>[7x]MQIQRHSFKWILYGFLCWMTSFVQAQTPTLTNATPAEGFIGEQVCFPVTFVNTGAPGYGPYVRLIVPTGFTFDNASFGGSIQTVQNLGVIVSGAPNNFVIDPIAQSNNNSTTSDTIFAPVGSTVILLEYPVGSMVQGGVSLISEVCMTVDPAATIGVPVDICTQGVYEFGDTPTGDNGPIAGANECEPIIPILFRFDKKVNGSDGVYNEVPGGGASLCHIHQYELNIDIAAAGTLNGPITITDVLPGELAYFGNISLPAGCSAVEPTVGGLGGTLTVTCNGSYPGSTANIDMQVTFDAAVSDTLDETICDDTDINNGATVNVPGNPSQSDTVVTHVEHVLLGHTNNTVSPVTIGQTVLYTIGAEITEYTAGLTAASITFIVPDGMIYNPASLTWAGTPVAAGNVVIVPGPGTGSTVTVDVHTQNGANILPCASPSLQYTADVNQTYANGDPVLSRDRLTHSSTLTYDLVEGATGCTTSAGTPIDVIDIFFQKTVNNSPPTGPGRNGQWWPGDVVQYRLELQIPSLDLDDVVITDFFPLPIHDVASLAATFGTDVRFDPATCWNTAPVTYTRDIPTNSLILDFGDVSDLVTGGCVDIVLLIDIPITTLPFADGLFHSNFMQVNSDNSTADNITNSALTLIQVGAPDLELTKGIVSSDNPNVTISPTVVPPDGNATDVSAGDQLFFDITIENVGGAPGYDVQVRDVAPPELTNCALVAPNPVVDGSNNALAFSGGFVGNTLTIDLVAPNDSIAFATAPNNNDLITVSYVCEAVAGIQAGTRFDNTAEVDWSSTRGGVKFPPVEDDANGRIADPTMNKVVDYIFPNYSNTNTQASIGEVVAYELQLNIPEGNMNNVTLVDQVDEGLAFVAVDSIVICNSSGSTNIITSIGGGFPAVQSGATITNLGANPQQQDRVLTLDFGNLQNLDTDNIEDTIKVYYRTIVINHVTNFDGERVRNRAVLSWDNPNTPGDRSSINDRAPFVTIVEPQLEISKSFTPDEVLPGNNSFVTLTVRNPGTSSAPAFDVSLTDILPTGMTFVSGFSAGGTASITTPPTNGGGTITAHWDTINVGEVYSITFEVQASSSITPCFTLTNCANLVWESIAEADEPNMPTAFSSNLGVQRTGNPGNLGGAANTYTQDSCADLDVVIDNTFDPFITANTPLCEGDRVVLTVQQYQGNVVRYNWTGPGVPAGFNNYELVLDPVTTADTGTYFVYVELDGCITDTSNFFSLQLRPKPVTPNINPGDTTICEGTSIQFSTSTIANDYTWTGPNGFTANSATTPLISPVTLADAGRYTLFTTNAQGCNSDPISSNLTVTPRPAQPSIASNTPICSNENIILTSSTSAITYQWMAPNGQDTITTNNTLTLEPNNPLYTAGNWTLVVFDANGCASQPSTAANVIINGTPIAPMTSNSGPICEGEDVTLMVNTVSSGTYAWYSDANLTNLVASTQNPVISGLLASNSPDTFYVQVSSNGCLSDTGFTVVQVNPNPAAVSPGYTPLCSGDTIFLFANATANIYNWTGPNGFVSNLENPFIANSAALNAGSYTVSITDANGCSNSGIVQVAVDERPVTPTITGNGPVCEGDNIQLNIGSYTGTTVQYTWSTPTGVVTTGVPSLNINNTTVADSGLYSVVVAVDGCTSLADSINIVVRPNPIAPNVPSNFSVCEGDGIALTTTTNANIYNWTGPNGFSSNSPNPTVISPASSANAGTYTLVVQDFNGCTSPAASTVVTVNAAPAQPSMTTNSPICNGADLVMSTSAAGNSYIWRAPNGADTTTASSTLTIVPTSSLYQSGNWTLSVVNAAGCVSPASIASAVEINSIPSTASAGNNGPVCTGTDASLSAGTVSGASYAWYTDAGTSNQFSTLQNPTVNNLTNDSTFYLLVTVNGCPSALDSTTVVVYPLTPSPS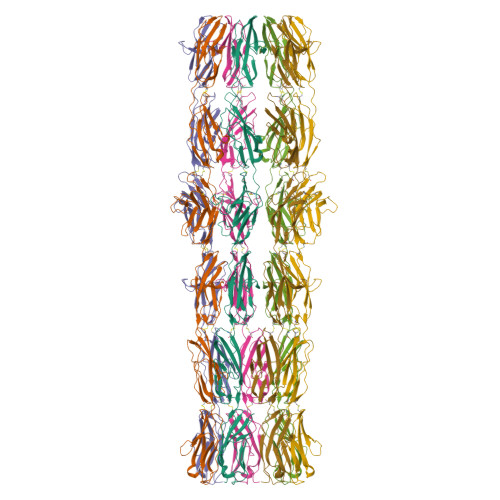LPANFAVCEGDDIALSTSTVASSYDWSGPNGFTSNAQNPVVITNATGSNAGVYTLSIVDGNGCSSADTSVQVTVNAAPTQPSMTTNSPICNGADLVMSTSAVGNSYIWRAPNGADTTTASSTLTIVPTSSLYQSGNWTLSVVNAAGCVSPASIASAVEINSIPSTASAGNNGPVCTGTDASLSAGTVSGASYAWYTDAGTSNQFSTLQNPTVNNLTNDSTFYLLVTVNGCPSALDSTTVVVYPLTPSPSLPADFAVCEGDDIALSTSTVASSYDWSGPNGFTSNAQNPVVITNATGSNAGVYTLSIVDGNGCSSADTSVQVTVNAAPAQPSMTTNSPICNGADLVMSTSATGNSYIWRAPNGADTTTASSTLTIVPTSSLYQSGNWTLSVVNAAGCVSPASIASAVEINSIPSTASAGNNGPVCTGTDASLSAGTVSGASYAWYTDAGTSNQFSTLQNPTVNNLTNDSTFYLLVTVNGCPSALDSTTVVVYPLTPSPSLPADFAVCEGDDIALSTSTVASSYDWSGPNGFTSNAQNPVVITNATGSNAGVYTLSIVDGNGCSSADTSVQVTVNAAPTQPSMTTNSPICNGADLVMSTSAVGNSYIWRAPNGADTTTASSTLTIAPTSSLYQSGNWTLSVVNAAGCVSPASVASMVTINNGTNPTAFNNGPVCRGDAVQLNTTTINNALYEWYSDAALTNLISTQQNPTVANITTDSTFYLVVTVNGCPSSAVATTVTLHPTPATPNIPANFVVCEGETIALSTSTVASSYNWTGPNGFTSNLQNPAVIQPATTADAGSYTLFIVDANGCQSADTSVVVGVNRGPAAPVLTNNSAICDGDTLLLSTTASADTFRWISPNGIDTITTVNSLMIVPTNGTYYQSGDWTLITQVANNCPSEPSAPSSVVINSSTAAPTAFNDGPVCVGGDVTLSTPSAPGAFYQWYTDAALTNLVATTASFTAINITQDSTFYLVVTVNGCTSPAGSTVVNVIGQPSAPNVPADFEVCEGDDIILGTTTIAASYSWTGPNGFTSNLQNPAAITNASLIDSGIYRLVVTYSNGCVSADTTVRVGVNSNPPVPNIVSNGPICFGDTLVLSSSTSCGQSQWIGPNGNSQSTLGTPGGSNVLWTIGSTTSIPMNNANYLPGNWYMICIDTVTGCRSESNTINVIINANPDTPAVFNDGPVCEGGNSNLSTATVSGASYAWYSDSSLTSLVSTAQNPMIVNISTDTTWYLVVTVNGCSSVAGSTTVIVHPTPVTPNVPANFAVCEGDNITLSTSTVASSYNWSGPNGFTSNVQNPVVITNATTSNAGVYTLSIIDGNGCESGDTAVTVTVDSIPATPVLSSNSAICFGDTLELSTTALATSYEWIAPDGSRITTGTNILSISSNNSLYQSGDWMLVTTNASGCTSMPSSVATVVINANPAQPAVFNDGPVCEGGNSNLSTATVSGASYAWYSDSSLTSLVSTAQNPMIVNISTDTTWYLVVTVNGCSSVAGSTTVIVHPTPATPNVPANFAVCEGDNITLSTSTVASSYNWSGPNGFTSNVQNPVVITNATTSNAGVYTLSIVDGNGCESGDTTVTVTVDSIPVTPVLSSNSAICFGDTLELSTTALATSYEWIAPDGSRITTGTNILSISSNNSLYQSGDWMLVTTNASGCTSMPSSVATVVINANPAQPAVFNDGPVCEGGNSNLSTATVSGASYAWYSDSSLTSLVSTAQNPMIVNISTDTTWYLVVTVNGCSSVAGSTTVIVYPTPATPNVPANFAVCEGDNITLSTSTVASGYNWSGPNGFTSNVQNPVVITNATASNAGVYTLSIVDGNGCESGDTTVTVTVNGNPPVATITSNSPICFGDTLTLSSSTNCGQSQWIGPNGNSSGTLGTPGGNNVLWTIGSTTNIPSTDVNYLSGDWYMICIDTITGCRSESNTITIEINPIPVVSAFNNGPICAGEDGELSATFITGASYRWYSDATLTTLISTSRTPIISSMMSSETYYVVATVNGCTSLADSTTIVVNPTPVIPNPTYTPLCQLDTLFLQANAVGPIATYWWTGPNGFTSHLENPVIPNIYPFNAGSYILTVTDSLGCEAVSTVEVTIYPKPQTPTIAHNAPFCEGTNDLTLTTQAYFGTDVRYIWTLPNGNLDTTFVPSLVLPNATVQDTGAYSLVVWIDGCLSLPAEEIIRIYPTPATPNVPADFAVCEGEAIVLTTTTNATSYFWTGPNGFQSNLQSPSVVNATLVDAGSYHLYVTNTWGCQSLDTSVQVTVNANPPIATITSNSPICFGDTLTLSSSTNCGQSQWIGPNGNSTGTLGTPGGNNVLWTIGSTTNIPSTDSNYLSGDWYMICIDTITGCRSESNTITIDINPIPSTPAAFNNGPICIGGTAQLSTTTVSGATYAWYADATLTTLVATNQNPTISNITTDSTFYIVVTVNGCSSLAGSTTVSTYPVPATPAVPADFAVCEGDNIVLSTTTVAAGYNWTGPNGFTSNLQNPSVVSASLVDSGTYTLFIIDANGCPSGDTSVQVSVHPNPVQPVLSSNSAICDGDSLVLSTTATATTYRWVAPDGADTLTTVNTLVILPSNAFYQDGNWTLMTMDANGCQSILSNPESVTIHSIPAAQAVFNNGPVCRGSSVNLSTSFISGATYEWYADAALTILVATSQNPTINNITTDSTFYLVITVNGCTSAAGATTVVVHPTPTTPNVPSNITVCEGDAIVLTTTTNASAYVWSGPNGFSSNQQSPTVINAATVVDSGKYSLYVIDANGCRSEDTSLQVVVNPTPTTPLIVSNNTPICEGSNIVLSANAGAAGTTYEWFNASNVSVGTGQTLTIVGATVADAGDYYVITTLNSCSSAASSTTTAIVDQVPSTAAFAGNDINLCNSFTTTLDATPPNSATGFWTTNSGATIANPNLANSAVYNLPTGTSTFYWTLSNGACIDFSVDSMVVEVTPASTDVADAGLDQNLCGQTSATLTAANPSTATGQWTQSASQAGQGIVITNPTNPNTTVTGLQQGNNYTFTWTLSNGNCTDYSTDMVQINVDVSPPDNAYAGVDILLCNQNTANLDAFVSQYGTGMWTSTSSATIIDPTLANTTVINLPQDTSVFVWTLSNGTCQNYSTDSVLVVVSTTTDTAEAGNNQVVCSVNALTLGATMPSSGFGTWSQTAAQAAQGVVIVDVNDPNTQVVGLNAGTTYAFTWTLSNGTCQDYSSDVTTISVNATPPDNAFAGNDINLCGVATTTNLAASVPTVAMGLWTTTSSATISNPTQPNSTVSGLSAGQNIFIWTLSNGTCQDYDSDTVIVTVTTPSSDVADAGLDSAYCAQSVVTLNAVAPSVGGGYWSQTPSQASLGAVIDNPTDTATTVSNLMPGVTYTFTWTLTNGGCVDYSSDQVLITIDVLPTNVAYAGEDTILCGGNAVQLDGLAPPIGTGFWTTNDTATIVTPVDPNSLVVNIAEDTTTYYWTLSNGACVDYSVDSVTVIISPASTDLAFAGYDEVLCGVDSIMLSAAVPTTSTGIWTQSAGQASQGIVITNPTNPNSSVTGIQAGQVYTFTWTLSTFGCANFSTDDVQYTINALPPEVAYAGPDIVLCTGNSVTMDANNPIFSTGVWSSNSSAVIVNPTLSNSNIVNIPTDTVAFYWSLSNGSCADYSIDTMLIIVTPTFSVDTANAGLDINLCNEDTAQLMAIAPNVATGRWTQPFNQSSAGVVITDPNAAMTTATGLQLDSTYTFTWSVSNGPCRDYDRDQVIVQVSTLPTDAAYAGEDFVICGIDTAIVSATAPSIGAGMWTTTTTATIVTPPSTRTELLNLSLGSNEFIWTLSNGACRDYSSDTIVITMDSAPIANADSFVVIYNSNGNTIDVTPNDGLNNNWVITISESIASGTLDNLGTGEFDLFLQDVLVDQRFIYQLCNPNCPAIYCDTALVTIDVQGGTECNFPNMITPNNDDANETFIVPCLDGLEGTKFAVYNRWGDLMYENDNYKNDWGGTHNGVPVPDATYFYIMELADGQRFQGFVEVRR> NVKINLNTYIEIIKLLLNQNRDIRLKFYGVLMAIGRRPVEVMKLSQFYIADKNHIRMEFIAKKRENNIINEVVFPVFADPELIINSIKEIRYMEQTENLTKELISSNLSYSYNR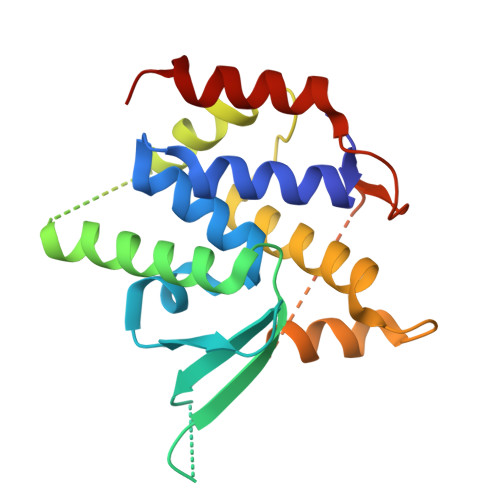LFRQIFNNIFAPEESVYFCRAIYCKFSYLAFAPKNMEMNYWITKVLGHEPNDITTAFHYNRYVLDNLNDKADNNLLKLLNQRIYTYVR>FACKTANGTAIPIGGGSANVYVNLAPVVNVGQNLVVDLSTQIFCHNDYPETITDYVTLQRGSAYGGVLSNFSGTVKYSGSSYPFPTTSETPRVVYNSRTDKPWPVALYLTPVSSAGGVAIKAGSLIAVLILRQTNNYNSDDFQFVWNIYANNDVVVPTGGCDVSARDVTVTLPDYRGSVPIPLTVYCAKSQNLGYYLSGTHADAGNSIFTNTASFSPAQGVGVQLTRNGTIIPANNTVSLGAVGTSAVSLGLTANYARTGGQVTAGNVQSIIGVTFVYQ[2x];>[2x]DLYFNPRFLADDPQAVADLSRFENGQELPPGTYRVDIYLNNGYMATRDVTFNTGDSEQGIVPCLTRAQLASMGLNTASVAGMNLLADDACVPLTTMVQDATAHLDVGQQRLNLTIPQAFMSNRARGYIPPELWDPGINAGLLNYNFSGNSVQNRIGGNSHYAYLNLQSGLNIGAWRLRDNTTWSYNSSDRSSGSKNKWQHINTWLERDIIPLRSRLTLGDGYTQGDIFDGINFRGAQLASDDNMLPDSQRGFAPVIHGIARGTAQVTIKQNGYDIYNSTVPPGPFTINDIYAAGNSGDLQVTIKEADGSTQIFTVPYSSVPLLQREGHTRYSITAGEYRSGNAQQEKPRFFQSTLLHGLPAGWTIYGGTQLADRYRAFNFGIGKNMGALGALSVDMTQANSTLPDDSQHDGQSVRFLYNKSLNESGTNIQLVGYRYSTSGYFNFADTTYSRMNGYNIETQDGVIQVKPKFTDYYNLAYNKRGKLQLTVTQQLGRTSTLYLSGSHQTYWGTSNVDEQFQAGLNTAFEDINWTLSYSLTKNA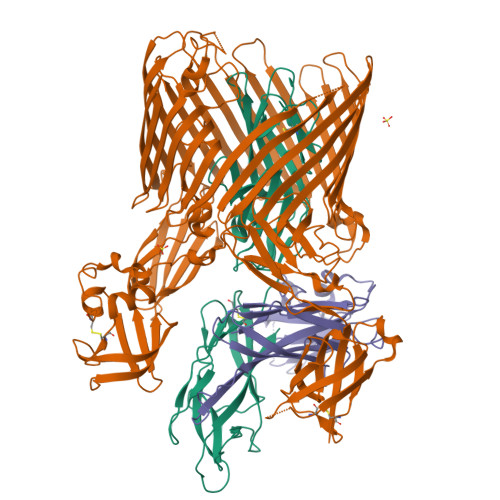WQKGRDQMLALNVNIPFSHWLRSDSKSQWRHASASYSMSHDLNGRMTNLAGVYGTLLEDNNLSYSVQTGYAGGGDGNSGSTGYATLNYRGGYGNANIGYSHSDDIKQLYYGVSGGVLAHANGVTLGQPLNDTVVLVKAPGAKDAKVENQTGVRTDWRGYAVLPYATEYRENRVALDTNTLADNVDLDNAVANVVPTRGAIVRAEFKARVGIKLLMTLTHNNKPLPFGAMVTSESSQSSGIVADNGQVYLSGMPLAGKVQVKWGEEENAHCVANYQLPPESQQQLLTQLSAECRSAWSHPQFEK;>GVALGATRVIYPAGQKQVQLAVTNNDENSTYLIQSWVENADGVKDGRFIVTPPLFAMKGKKENTLRILDATNNQLPQDRESLFWMNVKAIPSMDKSKLTENTLQLAIISRIKLYYRPAKLALPPDQAAEKLRFRRSANSLTLINPTPYYLTVTELNAGTRVLENALVPPMGESAVKLPSDAGSNITYRTINDYGALTPKMTGVMEHHHHHH[2x]N-[ethoxy(oxo)acetyl]-beta-D-glucopyranosylamine 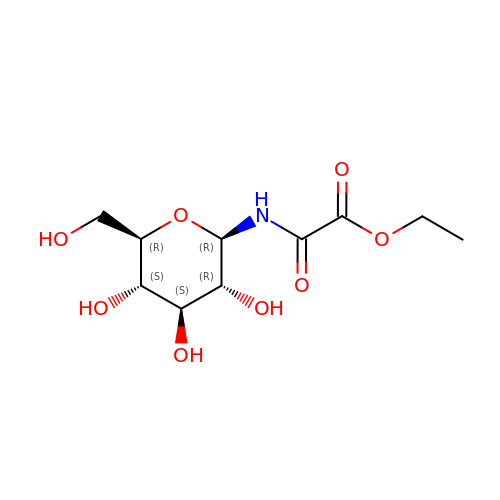| C10 H17 N O8 | TVQLSCFCYGZTNJ-XSEHCYKFSA-N>[2x]MNPAAEAEFNILLATDSYKVTHYKQYPPNTSKVYSYFECREKKTEN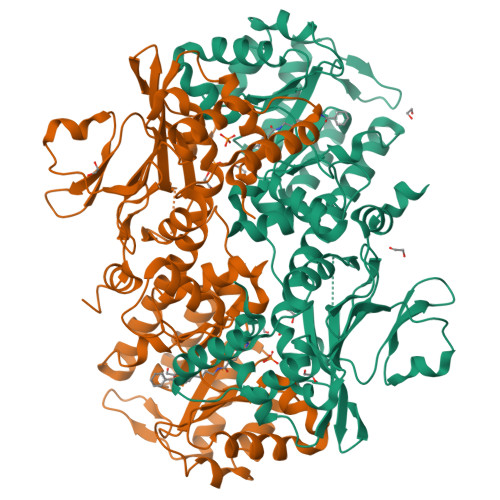SKLRKVKYEETVFYGLQYILNKYLKGKVVTKEKIQEAKDVYKEHFQDDVFNEKGWNYILEKYDGHLPIEIKAVPEGFVIPRGNVLFTVENTDPECYWLTNWIETILVQSWYPITVATNSREQKKILAKYLLETSGNLDGLEYKLHDFGYRGVSSQETAGIGASAHLVNFKRTDTVAGLALIKKYYGTKDPVPGYSVPAAEHSTITAWGKDHEKDAFEHIVTQFSSVPVSVVSDSYDIYNACEKIWGEDLRHLIVSRSTQAPLIIRPDSGNPLDTVLKVLEILGKKFPVTENSKGYKLLPPYLRVIQGDGVDINTLQEIVEGMKQKMWSIENIAFGSGGGLLQKLTRDLLNCSFKCSYVVTNGLGINVFKDPVADPNKRSKKGRLSLHRTPAGNFVTLEEGKGDLEEYGQDLLHTVFKNGKVTKSYSFDEIRKNAQLNIELEAAHHLEHHHHHHHH> GLGDLIEGVVEGVTRNALTPLTPANNLPDTQSSGPAHSKEIPALTAVETGATNPLVPSDTVQTRHVIQKRTRSESTVESFFARGACVAIIEVDNDAPTKRASKLFSVWKITYKDTVQLRRKLEFFTYSRFDMELTFVVTSNYTDANNGHALNQVYQIMFIPPGAPIPGKWNDYTWQTSSNPSVFYTYGAPPARISVPYVGIANAYSHFYDGFAKVPLAGQASTEGDSLYGAASLNDFGSLAVRVVNDHNPTKLTSKIRVYMKPKHVRVWCPRPPRAVPYYGPGVDYKDGLAPLPEKGLTTY;> MGAQVSSQKVGAHENSNRAYGGSTINYTTINYYRDSASNAASKQDFAQDPSKFTEPIKDVLIKTAPTLNSPNIEACGYSDRVMQLTLGNSTITTQEAANSVVAYGRWPEYIKDSEANPVDQPTEPDVAACRFYTLDTVTWRKESRGWWWKLPDALKDMGLFGQNMFYHYLGRAGYTVHVQCNASKFHQGALGVFAVPEMCLAGDSTTHMFTKYENANPGEKGGEFKGSFTLDTNATNPARNFCPVDYLFGSGVLAGNAFVYPHQIINLRTNNCATLVLPYVNSLSIDSMTKHNNWGIAILPLAPLDFATES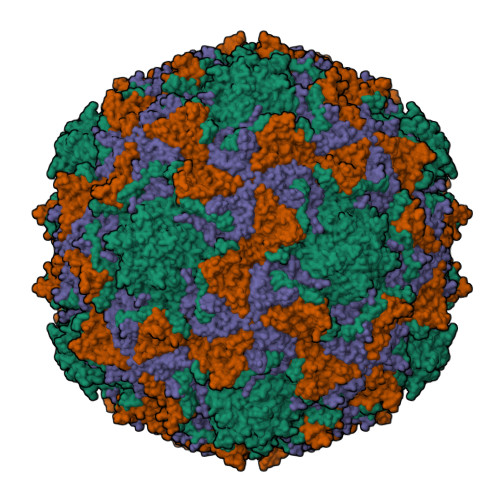STEIPITLTIAPMCCEFNGLRNITVPRTQ;> GLPVLNTPGSNQYLTADNYQSPCAIPEFDVTPPIDIPGEVRNMMELAEIDTMIPLNLTNQRKNTMDMYRVELNDAAHSDTPILCFSLSPASDPRLAHTMLGEILNYYTHWAGSLKFTFLFCGSMMATGKLLVSYAPPGAEAPKSRKEAMLGTHVIWDIGLQSSCTMVVPWISNTTYRLTINDSFTEGGYISMFYQTRVVVPLSTPRKMDILGFVSACNDFSVRLLRDTTHISQEAMPQ1-phenylurea | C7 H8 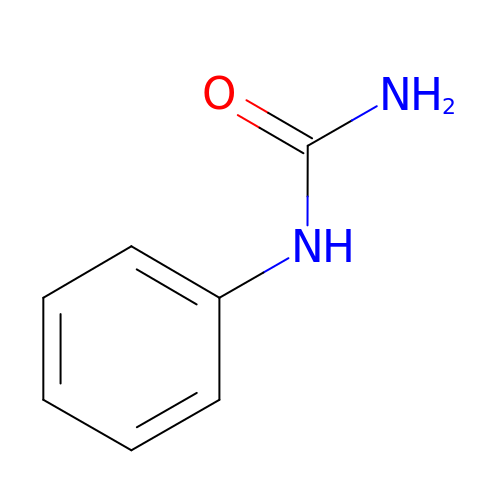N2 O | LUBJCRLGQSPQNN-UHFFFAOYSA-N> GFPVLNTPGSNQFMTSDDFQSPSAMPQFDVTPHMDIPGEVHNLMEIAEVDSVVPVNNIKVNLQSMDAYHIEVNTGNHQGEKIFAFQMQPGLESVFKRTLMGEILNYYAHWSGSIKLTFTFCGS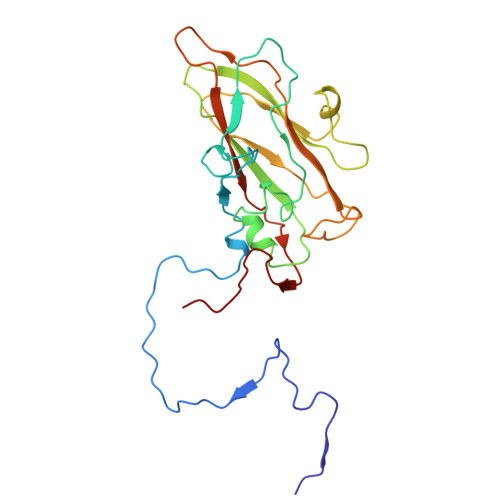AMATGKLLLAYSPPGADVPATRKQAMLGTHMIWDIGLQSSCVLCIPWISQTHYRLVQQDEYTSAGNVTCWYQTGIVVPPGTPNKCVVLCFASACNDFSVRMLRDTPFIGQTALLQ METHYL 1-(4-{[(2,4-DIAMINOPTERIDIN-6-YL)METHYL]AMINO}BENZOYL)PIPERIDINE-4-CARBOXYLATE 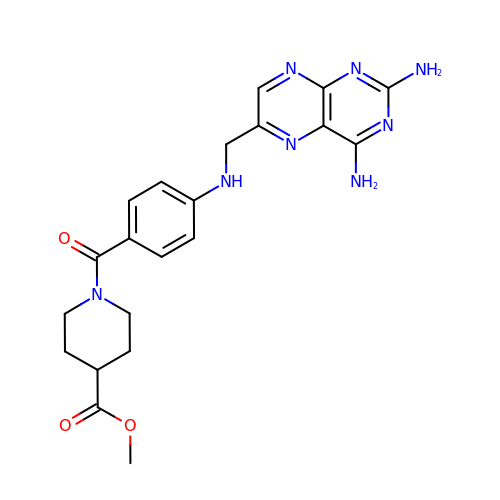| C21 H24 N8 O3 | NYNAFINLHQEHKU-UHFFFAOYSA-N> MNVTIYDVAREASVSMATVSRVVNGNPNVKPSTRKKVLETIERLGYRPNAVARGLASKKTTTVGVIIPDISNIFYAELARGIEDIATMYKYNIILSNSDQNQDKE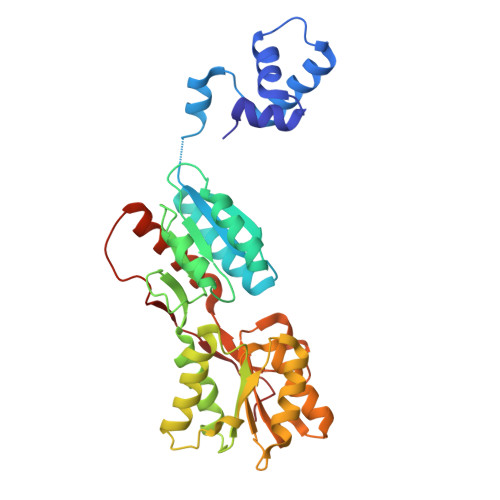LHLLNNMLGKQVDGIIFMSGNVTEEHVEELKKSPVPVVLAASIESTNQIPSVTIDYEQAAFDAVQSLIDSGHKNIAFVSGTLEEPINHAKKVKGYKRALTESGLPVRDSYIVEGDYTYDSGIEAVEKLLEEDEKPTAIFVGTDEMALGVIHGAQDRGLNVPNDLEIIGFDNTRLSTMVRPQLTSVVQPMYDIGAVAMRLLTKYMNKETVDSSIVQLPHRIEFRQSTK>[4x]MSKLIVPQWPQPKGVAACSSTRIGGVSLPPYDSLNLGAHCGDNPDHVEENRKRLFAAGNLPSKPVWLEQVHGKDVLKLTGEPYASKRADASYSNTPGTVCAVMTADALPVLFCNRAGTEVAAAHAGWRGLCAGVLEETVSCFADNPENILAWLGPAIGPRAFEVGGEVREAFMAVDAKASAAFIQHGDKYLADIYQLARQRLANVGVEQIFGGDRCTYTENETFFSYRRDKTTGRMASFIWLILEHHHHHH

YfiH is a PG-editing factor whose absence causes misincorporation of l-Ser instead of l-Ala into peptide stems, but its mechanistic function is unknown. Here, we report the crystal structures of substrate-bound and product-bound YfiH, showing that YfiH is a cytoplasmic amidase that controls the incorporation of the correct amino acid to the nucleotide precursors by preferentially cleaving the nucleotide precursor by-product UDP–MurNAc–l-Ser. Our results show that YfiH forms an extended L-shaped binding groove for the UDP-MurNAc-monopeptide and is a cytoplasmic amidase specific for hydrolyzing UDP–MurNAc–l-Ser, a noncanonical reaction by-product from the MurC reaction. Our results showing YfiH as an l-Ser-specific UDP-MurNAc-monopeptide amidase therefore uncover a bacterial control mechanism to ensure only the presence of the specific amino acid in the peptide assembly pathways by removing unwanted UDP-MurNAc-monopeptide byproducts from the MurC reactions.

Based on the genetic observation that the absence of yfiH leads to the misincorporation of l-Ser instead of l-Ala into PG, our crystallographic results suggest that YfiH may prevent the incorporation of l-Ser by specifically hydrolyzing UDP–MurNAc–l-Ser (UMS) as the preferred substrate. The cocrystal structure, determined at a 1.86-Å resolution, shows that Gln69 indeed forms a hydrogen bond with the side chain hydroxyl of l-Ser of the substrate, whose carboxylic group forms a bidentate salt bridge with Arg235. Moreover, the measured specific activity of YfiH on UMS was more than 10-fold greater than on UMA. Removing the side chain of Arg235 significantly decreased the hydrolytic activity. The results show that the activity for UMS, but not for UMA, was significantly reduced in both the Q69A and Q69M mutants and that the activity for UMA was affected in the Q69A mutant. Overall, these results demonstrate that Gln69 is the specificity determinant residue.> MTNIQTQLDNLRKTLRQYEYEYHVLDNPSVPDSEYDRLFHQLKALELEHPEFLTSDSPTQRVGAKPLSGFSQIRHEIPMLSLDNAFSDAEFNAFVKRIEDRLILLPKPLTFCCEPKLDGLAVSILYVNGELTQAATRGDGTTGEDITANIRTIRNVPLQLLTDNPPARLEVRGEVFMPHAGFERLNKYALEHNEKTFANPRNAAAGSLRQLDPNITSKRPLVLNAYGIGIAEGVDLPTTHYARLQWLKSIGIPVNPEIRLCNGADEV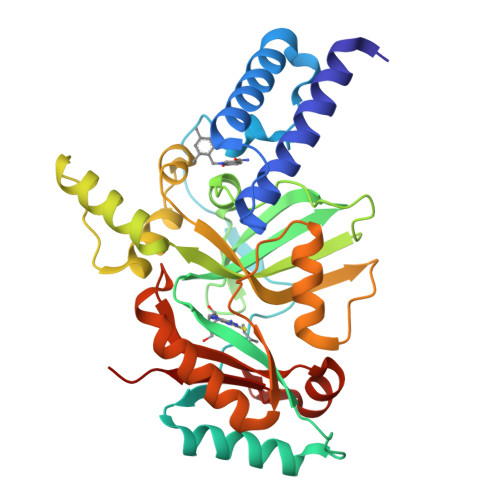LGFYRDIQNKRSSLGYDIDGTVLKINDIALQNELGFISKAPRWAIAYKFPA> MTDQFERNNIRNNEVAAEQSIQSNNFGGLNTLASPLNVPYQDSPLLLNTTVDTSGQVYKRKGTRITYTTTGTSTGCYITGFTSGLAYQFQVAKRGRDILLFQTTNDVTSLLLTKSNVWDTRAEAVRPSVVTTSEVTPRVIFATGVNKPVQLLFVEQQTTQTANGTSVVFSSADRFVNASTANCLVYVNRVLVSAPSFSYNAGTKQLTVSNLGSTVIGDVIDLVSVTWQWWAESQFWYGDRFFGSTTRFNSVSFDRVVKIPTSITTQNNGSDPYYRMRLYKQSNRTGSPNLNEVVQPQLADDWAFSDGSIYNYSVNDYPNPSPFWVVFGALVGGGQPSTVYFSRRRGLGFANGTSVQASKIDVVVNGVQRTPIYTPGSAPDSVYRNYYTYFADTTGAATGTSSTSLVNGIFFDAIPLGLATNDTVEASNNTNIHIGSASIATRYNYNDGSYIPAFGLGDFADYLNGYYPSVVTFFQGRLVFGGFPHRPLQVVFSNVNDNITPGRYYNSFSITDDNTALSSAFDIILNSRPDDRVVALIEWQSSLFILTRQAVFRANGGSSILSSTNRVISYVSSNGCTNSRCIVRTDFNVMYLSDTGVYNINPLVENGEYTVKELSIKIRDKFGVTREPVYEELPWMAYDSVNKQVLLGYPDVGQTNTSRYVYVYNTYRESWTEYNTPCGFNIWSTTEYTDRLLGTSVCSILYTTTSSGTPSNFIIIRWNASLYIDFIQRKTHNGSSYELTTQPAVTHTTNVNQRRYGVNFTLTRQNTAFT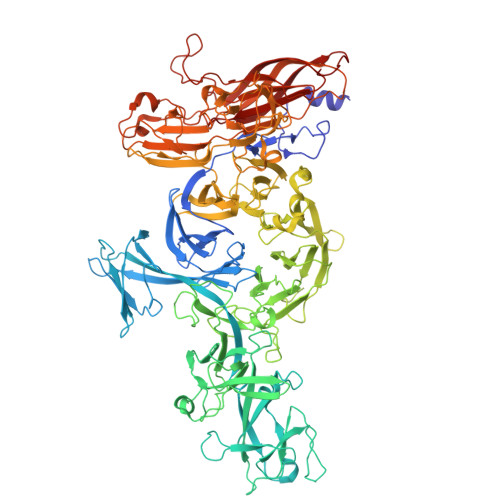INPVTTVNDLYVTLDGTLLTPNVDYIKEETGYIYLLSTFSTGQTLKIASSPEGNTTPNSWYTVYVNNIRQVSPTPSAGTFTLGATNGDIINWGVNYLTIYTTPQFLWNSLGNFKRTQHAYLFLDNRDGVGVYVASDVNNGQDINQLTELYRVPINFNLSVMYNNQLDGSTSYDVMGYDSMYWDEGVFDVSSPYDQYQPYQTLKIPITGIGYAFQMLIWNHSDEYFKLGGYQIIAKQKGKRHIGRY The human AAA-ATPase Bcs1L translocates the fully assembled Rieske iron-sulfur protein (ISP) precursor across the mitochondrial inner membrane, enabling respiratory Complex III assembly. Bcs1L is a membrane-bound oligomer, with each subunit consisting of an N-terminal TM segment, a middle Bcs1-specific domain, and a C-terminal AAA domain that is highly distinct, forming a clade of its own in the broad AAA protein family. Here, we captured Bcs1L conformations by cryo-EM during active ATP hydrolysis in the presence or absence of ISP substrate. In contrast to the threading mechanism widely employed by AAA proteins in substrate translocation, subunits of Bcs1L alternate uniformly between ATP and ADP conformations without detectable intermediates that have different, co-existing nucleotide states, indicating that the subunits act in concert.

Further 3D classifications to look for different conformations yielded only two distinct conformations, with 3/4 classes (322,765 particles, approximately 95% of the selected particles after the 2D classification) resembling the ATPγS state with disordered TM cavity (ATP state-1), and a minor population (5%, 15,083 particles) resembling the Apo/ADP state. Using the best class of particles after 3D classification (class 3 in pink), which contained 200,466 particles and did not give detectable tetradecamer signals, the map was refined to 3.77 Å resolution with C1 symmetry and to 3.13 Å with C7 symmetry. Global superposition of the refined mBcs1L-ATP heptamer model with the reported model of mBcs1L with bound ATPγS gave a rms deviation of 0.644 Å for 1,743 aligned CA atoms with the ATP-bound Bcs1L slightly expanded in diameter. In both C1 and C7 maps, the nucleotide-binding sites are exceptionally well-defined in the density, with local resolutions estimated at 3.5 and 3.0 Å, respectively, exceeding the global resolutions of the reconstructed maps and providing confidence in the assignment of nucleotide state. The AAA ATPase regions are very much the same, but they differ substantially in the TM region and the Bcs1-specific region when compared to the ATPγS-state and to each other. The Matrix-seal in the ATP state-1 has the widest opening, as the β-sheets I tilts further away from MIM and the seal loops become too flexible to trace in the density map (middle). The conformation of β-Sheet II in ATP state-1 is partially extended with the density at the tip being less well-defined (top). In the ATP state-1 conformation, both Matrix-seal and IMS-seal are open transiently, allowing passage of ISP-ED.

>[7x]MPFSDFVLALKDNPYFGAGFGLVGVGTALAMARKGAQLGLVAFRRHYMITLEVPARDRSYAWLLSWLTRHSTRTQHLSVETSYLQHESGRISTKFEFIPSPGNHFIWYQGKWIRVERNRDMQMVDLQTGTPWESVTFTALGTDRKVFFNILEEARALALQQEEGKTVMYTAVGSEWRTFGYPRRRRPLDSVVLQQGLADRIVKDIREFIDNPKWYIDRGIPYRRGYLLYGPPGCGKSSFITALAGELEHSICLLSLTDSSLSDDRLNHLLSVAPQQSLVLLEDVDAAFLSRDLAVENPIKYQGLGRLTFSGLLNALDGVASTEARIVFMTTNYIDRLDPALIRPGRVDLKEYVGYCSHWQLTQMFQRFYPGQAPSLAENFAEHVLKATSEISPAQVQGYFMLYKNDPMGAVHNIESLRPRDHHHHHH OTS964 | C23 H24 N2 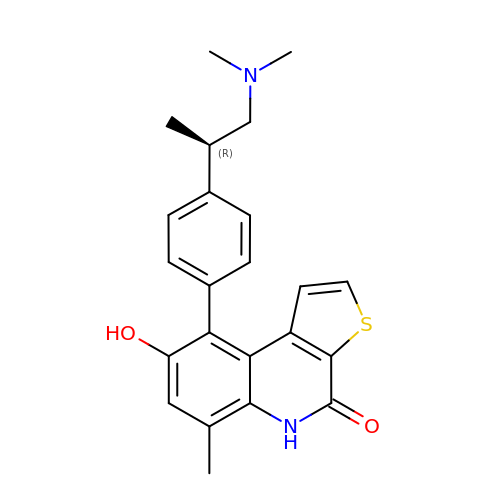O2 S | XCFRUAOZMVFDPQ-AWEZNQCLSA-N>MRTFDLEEKLQTNKYNANFVTFMEGKDFNVEYIQRGGLRDPLIFKNSDGLGIKMPDPDFTVNDVKMCVGSRRMVDVMDVNTQKGIEMTMAQWTRYYETPEEEREKLYNVISLEFSHTRLENMVQRPSTVDFIDWVDNMWPRHLKESQTESTNAILEMQYPKVQKYCLMSVRGCYTDFHVDFGGTSVWYHIHQGGKVFWLIPPTAHNLELYENWLLSGKQGDIFLGDRVSDCQRIELKQGYTFVIPSGWIHAVYTPTDTLVFGGNFL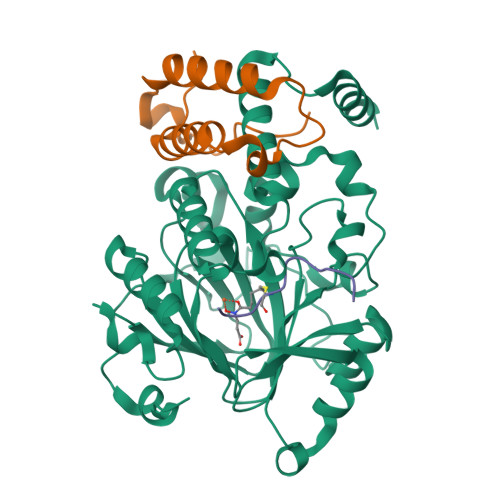HSFNIPMQLKIYSIEDRTRVPNKFRYPFYYEMCWYVLERYVYCITNRSHLTKDFQKESLSMDME[2x];>[2x]MQVHLTHFELEGLRCLVDKLESLPLHKKCVPTGIEDEDALIADVKILLEELASSDPKLALTGVPIVQWP;>[2x]APATGGVCKPHRY>[2x]GSMSGNGNAAATAEENSPKMRVIRVGTRKSQLARIQTDSVVATLKASYPGLQFEI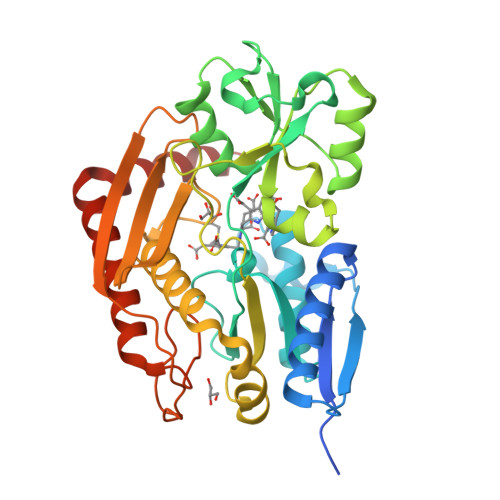IAMSTTGDKILDTALSKIGEKSLFTKELEHALEKNEVDLVVHSLKDLPTVLPPGFTIGAICKRENPHDAVVFHPKFVGKTLETLPEKSVVGTSSLRRAAQLQRKFPHLEFRSIRGNLNTWLRKLDEQQEFSAIILATAGLQRMGWHNRVGQILHPEECMYAVGQGALGVEVRAKDQDILDLVGVLHDPETLLRCIAERAFLRHLEGGCSVPVAVHTAMKDGQLYLTGGVWSLDGSDSIQETMQATIHVPAQHEDGPEDDPQLVGITARNIPRGPQLAAQNLGISLANLLLSKGAKNILDVARQLNDAH6-cyclopropyl-8-fluoranyl-2-[2-(hydroxymethyl)-3-[1-methyl-5-[[5-(4-methylpiperazin-1-yl)pyridin-2-yl]amino]-6-oxidanylidene-pyridin-3-yl]phenyl]isoquinolin-1-one 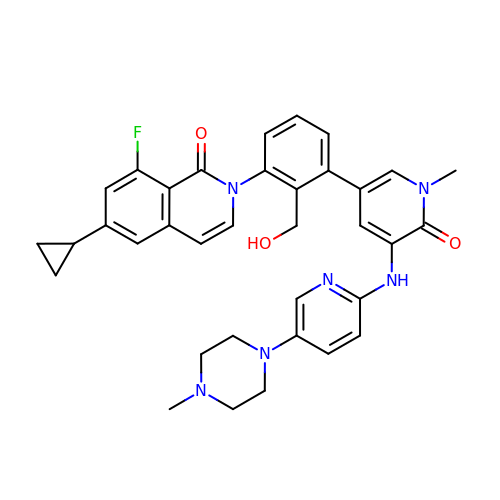| C35 H35 F N6 O3 | ZTUJNJAKTLHBEX-UHFFFAOYSA-N> HMASMTGGQQMGRGSDFGDIEERGKI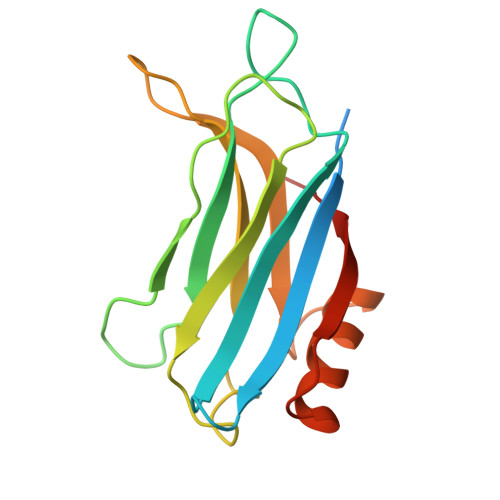LVSLMYSTQQGGLIVGIIRCVHLAAMDANGYSDPFVKLWLKPDMGKKAKHKTQIKKKTLNPEFNEEFFYDIKHSDLAKKSLDISVWDYDIGKSNDYIGGCQLGISAKGERLKHWYECLKNKDKKIERWHQLQNENH>[4x]HHHHHHSSGLVPRGSHMASMSKVGINGFGRIGRLVLRRLLEVKSNIDVVAINDLTSPKILAYLLKHDSNYGPFPWSVDFTEDSLIVDGKSIAVYAEKEAKNIPWKAKGAEIIVECTGFYTSAEKSQAHLDAGAKKVLISAPAGEMKTIVYNVNDDTLDGNDTIVSVASATTNCLAPMAKALHDSFGIEVGTMTTIHAYTGTQSLVDGPRGKDLRASRAAAENIIPHTTGAAKAIGLVIPELSGKLKGHAQRVPVKTGSVTELVSILGKKVTAEEVNNALKQATTNNESFGYTDEEIVSSDIIGSHFGSVFDATQTEITAVGDLQLVKTVAWYDNEYGFVTQLIRTLEKFAKL

Glyceraldehyde-3-phosphate dehydrogenase (GAPDH) is a highly conserved enzyme involved in the ubiquitous process of glycolysis and presents a loop (residues 208–215 of Escherichia coli GAPDH) in two alternative conformations (I and II). In the presence of inorganic phosphate (Pi), GAPDH catalyzes the conversion of D-glyceraldehyde-3-phosphate (G3P) to 1,3-diphosphoglycerate (BPG), accompanying the reduction of NAD+ to NADH. All the structures reported in this paper have four subunits: O, P, Q, and R. Each subunit contained two domains: the C-terminal catalytic domain and the N-terminal NAD+-binding domain. Two anion recognition sites, “Ps” and “Pi”, bind the C3 phosphate of G3P and inorganic phosphate, respectively.

The activity of EcGAPDH1 mutants was measured in the buffer with 40 mM triethanolamine, 50 mM K2HPO4 at pH 10.0, and 0.2 mM EDTA at 50 °C. The results showed that the enzymatic activity of C150A and C150A+H177A was abolished. In C150A.NAD.PO4, all the subunits have two phosphate-binding sites. Phosphate in the “new Pi” site is around the catalytic amino acid Cys150. Phosphate in the “new Pi” site is around the active amino acid Cys150. This phosphate will lose the occlusion from the side chain of cystine after mutation. Secondly, the catalytic cavity increased almost 6 Å3 after the mutant cysteine to alanine, which allows the “new Pi” site to occupy the phosphate.> MGPYGQEMYAFRSEERFKSPPILPPHLLQVILNKDTNISCDPALLPEPNHVMLNHLYAL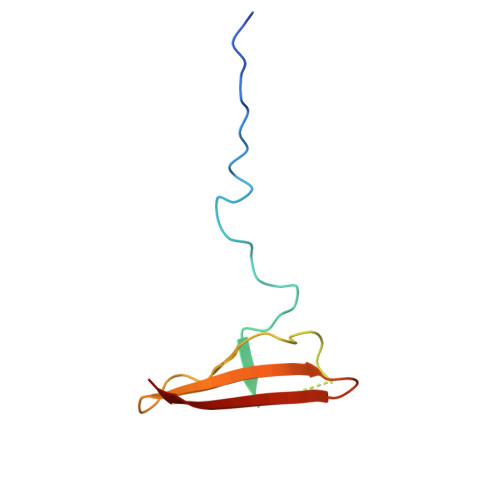SIKDSVMVLSATHRYKKKYVTTLLYKPI> MSNELRLEDNYVPTSDTLVVFKQLMKLPVTVLYDLTLSWFAKFGGSFDGDIYLLTETLDLLIEKGVRRNVIVNRILYVYWPDGLNVFQLAEIDCHLMISKPEKFKWLPSKALRGDGKPYVVKLQPAKFIENLQTDLAKIYHCHVYMFKHPSLPVLITRIQLFDSNNLFLSTPNIG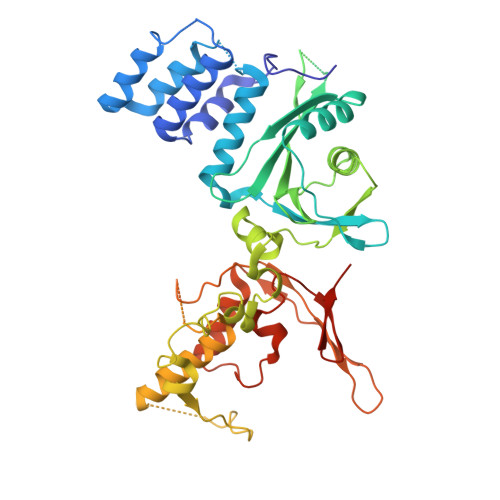SINKESLYNKLDKFQGKPLISRRPYYVAFPLNSPIIFHSVDKDIYARLVLQSISRTISERETIIFKPVQKIPVKSIHNIMTLLGPSRFAESMGPWECYASANFERSPLHDYKKHQGLTGKKVMVREFDDSFLNDDENFYGKEEPEIRRLRLEKNMIKFKGSANGVMDQKYNDLKEFNEHVHNIRNGKKNEDSGEPVYISRYSSLVPIEKVGFTLKNEINSRIITIKLKFNGNDIFGGLHELCDKNLINIDKVPGWLAGENGSFSGTIMNGDFQREQVAKGGLLENLYFQ>APADNAADARPVDVSVSIFINKIYGVNTLEQTYKVDGYIVAQWTGKPRKTPGDKPLIVENTQIERWINNGLWVPALEFINVVGSPDTGNKRLMLFPDGRVIYNARFLGSFSNDMDFRLFP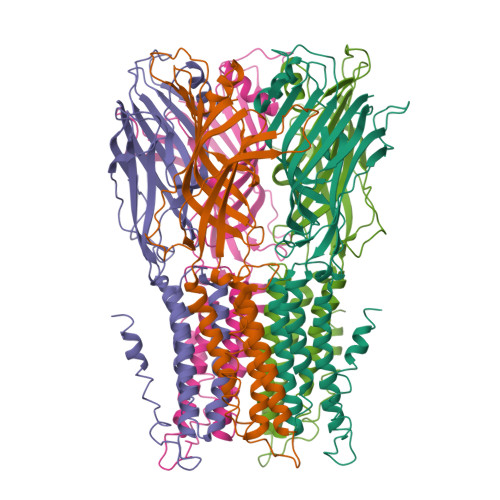FDRQQFVLELEPFSYNNQQLRFSDIQVYTENIDNEEIDEWWIRKASTHISDIRYDHLSSVQPNQNEFSRITVRIDAVRNPSYYLWSFILPLGLIIAASWSVFWLESFSERLQTSFTLMLTVVAYAAYTSNILPRLPYTTVIDQMIIAGYGSIFAAILLIIFAHHRQANGVEDDLLIQRCRLAFPLGFLAIGCVLVIRGITL[10x]> NRADDARNEVLRGNLVRAELWYRQIQENDQLKLENKGLKTDLREKEEELQGLKDDVEKLTADAELQRLKNERHE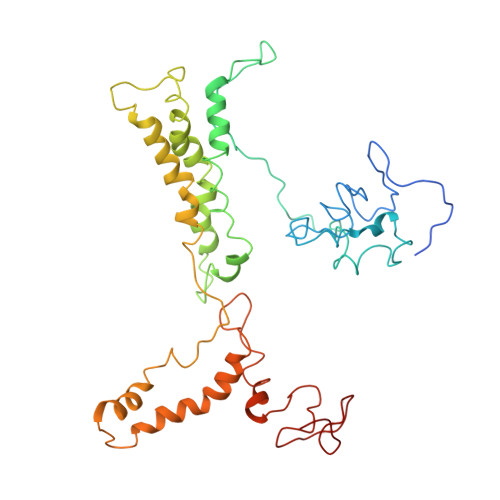EAELERLKSERHDHDKKEAERKALEDKLADKQEHLNGALRYINEKEAERKEKEAEQKKLKEEKQISDASRQGLRRDLDASREAKKQVEKDLANLTAELDKVKEEKQISDASRQGLRRDLDASREAKKQVEKGLANLTAELDKVKEEKQISDASRQGLRRDLDASREAKKQVEKALEEANSKLAALEKLNKELEESKKLTEKEKAELQAKLEAEAKALKEQLAKQAEELAKLRAEKASDSQTPDAKPGNKAVPGKGQAPQAGTKPNQNKAPMKETKRQLPSTG>[4x]MSLEIIKTGLAAFGMSGQVFHAPFISTNPHFELYKIVERSKELSKERYPQASIVRSFKELTEDPEIDLIVVNTPDNTHYEYAGMALEAGKNVVVEKPFTSTTKQGEELIALAKKKGLMLSVYQNRRWDADFLTVRDILAKSLLGRLVEYESTFARYRNFIKPNTWKETGESGGGLTYNLGSHLIDQAIQLFGMPEAVFADLGILREGGKVDDYFIIHLLHPSLAPNVKITLKASYLMR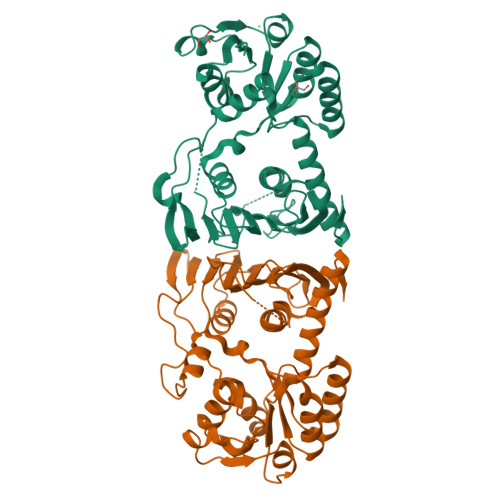EAEPRFALHGTLGSYVKYGVDKQEAALLAGEIPERPNWGEESEQEWGLLHTEINGKEICRKYPGIAGNYGGFYQNIYEHLCLGQPLETHAQDILNVIRIIEAAYQSHRENKIVNLKEGHHHHHH> MQLTDFKALTFDCYGTLIDWETGIVNALQPLAKRTGKTFTSDELLEVFGRNESPQQT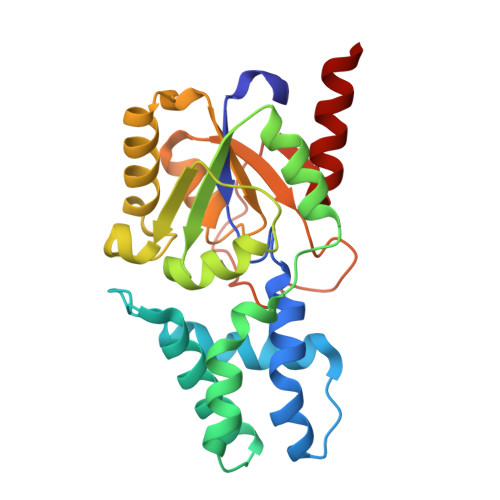ETPGALYQDILRAVYDRIAKEWGLEPDAAEREEFGTSVKNWPAFPDTVEALQYLKKHYKLVILSNIDRNEFKLSNAKLGVEFDHIITAQDVGSYKPNPNNFTYMIDALAKAGIEKKDILHTAESLYHDHIPANDAGLVSAWIYRRHGKEGYGATHVPSRMPNVDFRFNSMGEMAEAHKQALKG> NLYFQSARFAL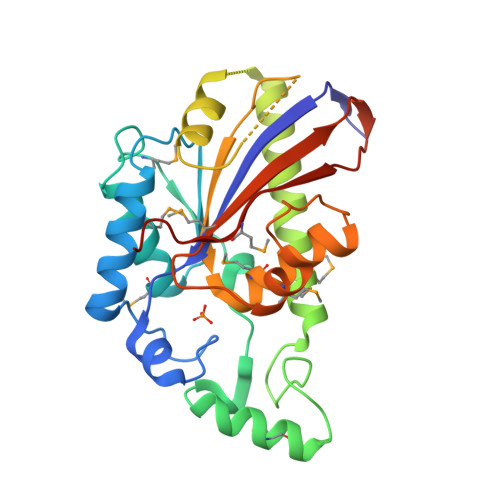TVVRHGETRFNKEKIIQGQGVDEPLSETGFKQAAAAGIFLNNVKFTHAFSSDLMRTKQTMHGILERSKFCKDMTVKYDSRLRERKYGVVEGKALSELRAMAKAAREECPVFTPPGGETLDQVKMRGIDFFEFLCQLILKEADQKEQFSQGSPSNCLETSLAEIFPLGKNHSSKVNSDSGIPGLAASVLVVSHGAYMRSLFDYFLTDLKCSLPATLSRSELMSVTPNTGMSLFIINFEEGREVKPTVQCICMNLQDHLNGLTETR>MRRSGNYNPSRWDVNFIQSLLSDYKEDKHVIRASELVTLVKMELEKETDQIRQLELIDDLQRMGLSDHFQNEFKEILSSIYLDHHYYKNPFPKEERDLYSTSLAFRLLREHGFQVAQEVFDSFKNEEGEFKESLSD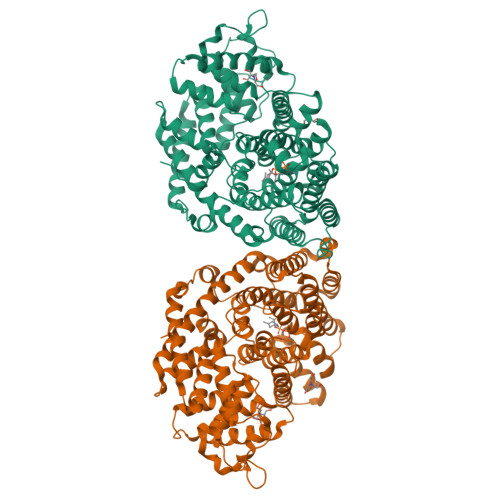DTRGLLQLYEASFLLTEGETTLESAREFATKFLEEKVNEGGVDGDLLTRIAYSLDIPLHWRIKRPNAPVWIEWYRKRPDMNPVVLELAILDLNIVQAQFQEELKESFRWWRNTGFVEKLPFARDRLVECYFWNTGIIEPRQHASARIMMGKVNALITVIDDIYDVYGTLEELEQFTDLIRRWDINSIDQLPDYMQLCFLALNNFVDDTSYDVMKEKGVNVIPYLRQSWVDLADKYMVEARWFYGGHKPSLEEYLENSWQSISGPCMLTHIFFRVTDSFTKETVDSLYKYHDLVRWSSFVLRLADDLGTSVEEVSRGDVPKSLQCYMSDYNASEAEARKHVKWLIAEVWKKMNAERVSKDSPFGKDFIGCAVDLGRMAQLMYHNGDGHGTQHPIIHQQMTRTLFEPFA[2x]>MGRKKIQIQRITDERNRQVTFTKRKFGLMKKAYELSVLCDCEIALIIFNHSNKLFQYASTDMDKVLLKYTEYNEPHESRTNADIIET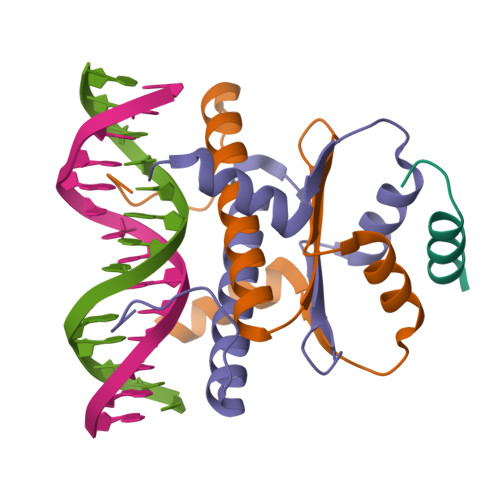LRKKGFNG[2x];> WGSGEVKLRLQEFLLSKS> MKIFIVGSTGRVGKSLLKSLSTTDYQIYAGARKVEQVPQYNNVKAVHFDVDWTPEEMAKQLHGMDAIINVSGSGGKSLLKVDLYGAVKLMQAAEKAEVKRFILLSTIFSLQPEKWIGAGFDALKDYYIAKHFADLYLTKETNLDYTIIQPGALTE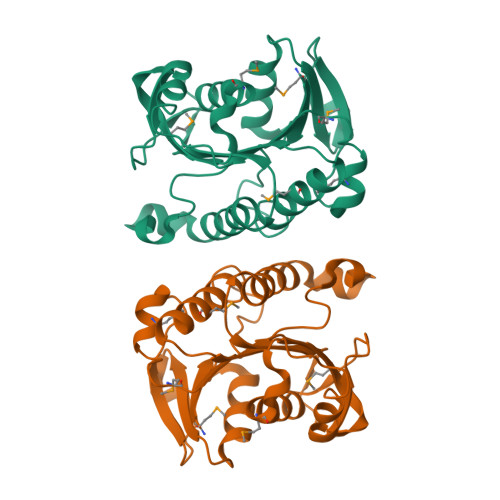EEATGLIDINDEVSASNTIGDVADTIKELVMTDHSIGKVISMHNGKTAIKEALESLLEHHHHHH> GAG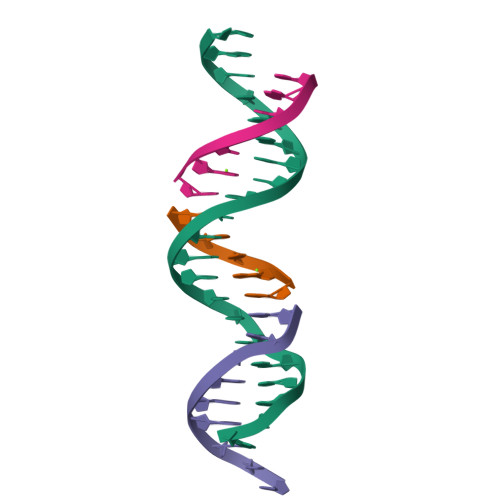CAGACAAGACTCCACTCA;> AGTCT;> TCTGAGTGG;> TGTCTGC>MAKNRRDRNSWGGFSEKTYEWSSEEEEPVKKAGPVQVLIVKDDHSFELDETALNRILLSEAVRDKEVVAVSVAGAFRKGKSFLMDFMLRYMYNQESVDWVGDYNEPLTGFSWRGGSERETTGIQIWSEIFLINKPDGKKVAVLLMDTQGTFDSQSTLRDSATVFALSTMISSIQVYNLSQNVQEDDLQHLQLFTEYGRLAMEETFLKPFQSLIFLVRDWSFPYEFSYGADGGAKFLEKRLKVSGNQHEELQNVRKHIHSCFTNISCFLLPHPGLKVATNPNFDGKLKEIDDEFIKN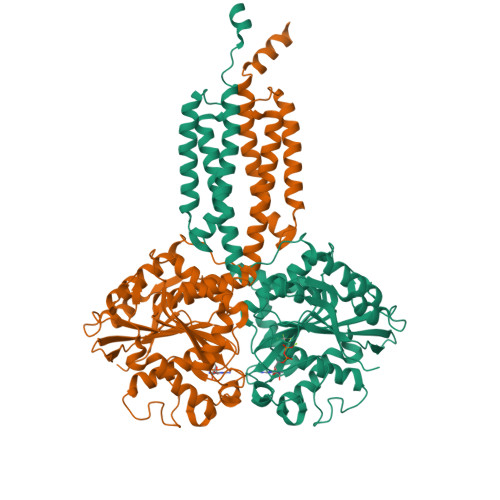LKILIPWLLSPESLDIKEINGNKITCRGLVEYFKAYIKIYQGEELPHPKSMLQATAEANNLAAVATAKDTYNKKMEEICGGDKPFLAPNDLQTKHLQLKEESVKLFRGVKKMGGEEFSRRNYLQQLESEIDELYIQYIKHNDSKNIFHAARAAALEHHHHHH[2x]>MTDQTTVVDITSAPLTPKEKLDLYCEALCDGFNKTQAYIKAGFSAPHAQRNVAPY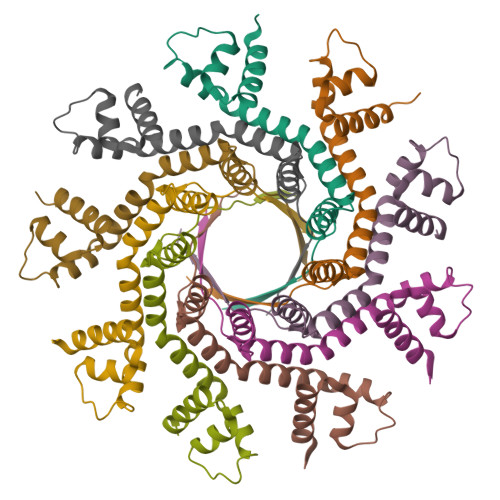HRKNAEYIQAYISERIGSDAPAARKVVLEIMNDPNEKGGIRLKAAQDILDRAGFGAKQKIELTTKDVADLTTEDIKNELAKLFNDEPELAKVVAFPINHSKS[81x]> DHYNCVSSGGQCLYSACPIFTR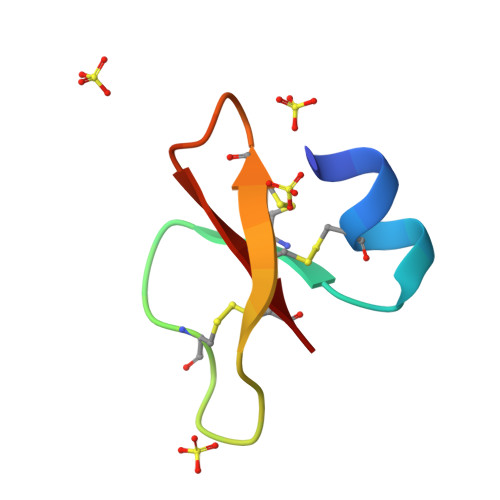IQGTCYRGRARCCR>[2x]VSFSVPGLVVEDMSNSRWPAQINGLVVRGNEAQVVHFQNGRCTTEGTLLGTTTLSINSICGLRGLSVSQASVRGAPALTEEMPPLEDEVADGAAATYTLARAADTTLWLRVEEPDGRPYDIFGDQPAPLGTPDFTAVIVGTAIRPRTASGAYLHDAYVDTTPGDADFTPSTGNTKIVLRGGGSGHVGQGHYWQFRPIAVEGGG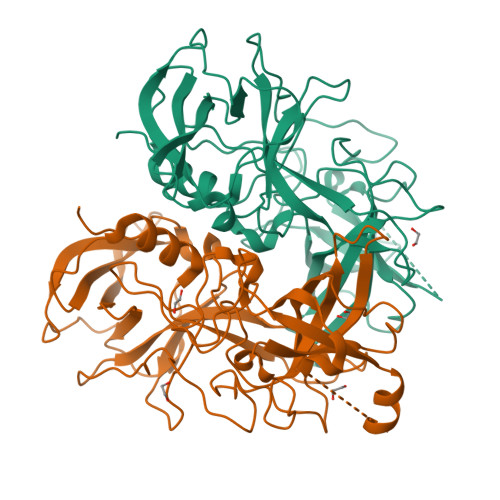SRPQYQEYNLPDYAGPTASNHDLAPPVAPRMPGELLLLFESDMPVWDNGAGAAPAQKIHCLLPNEFITHLFDLQAPALAEAALLRYVHPDSGRTLFECKLYREGYMVVAAPAGRLNFPLDGYFRFDSWVSAFYILSPV>MSGSEELLEELRELLERLQELLELIEQGKITPEQLREAIALLIEVLQILYEALRELAEQLQRLREELGS[2x]

Here, we computationally designed monomeric and homo-oligomeric miniproteins binding with high affinity to the MERS-CoV spike (S) glycoprotein, the main target of neutralizing antibodies and vaccine development. MERS-CoV S comprises an S1 subunit, which mediates binding to sialosides via the N-terminal domain (NTD) and to the dipeptidyl-peptidase 4 entry receptor (DPP4) via the receptor-binding domain (RBD), as well as an S2 subunit which promotes virus and host membrane fusion to initiate infection,12–17. We show that these miniproteins broadly neutralize a panel of MERS-CoV S variants, spanning the known antigenic diversity of this pathogen, by targeting a conserved site in the receptor-binding domain (RBD). The miniproteins directly compete with binding of the DPP4 receptor to MERS-CoV S, thereby blocking viral attachment to the host entry receptor and subsequent membrane fusion.

Based on our previous success in designing a homotrimeric, pan-variant SARS-CoV-2 inhibitor, designated TRI2–224–27, we set out to engineer homotrimeric versions of cb3 to enable simultaneous engagement of all three RBDs within a MERS-CoV S trimer and enhance potency and breadth further through avidity. 12 trimeric cb3 constructs were designed, consisting of 6 oligomerization domains with both N- and C-terminal fusions for each oligomerization domain (denoted with prefix ‘n’ or ‘c’ to describe the position of the miniprotein relative to the trimerization domain). Two of these failed to express (nTrimer3 and nTrimer4). Evaluation of neutralizing activity against the MERS-CoV EMC/2012, Jordan/2012 and United Kingdom/2012 pseudoviruses revealed that trimeric cb3 miniproteins were endowed with at least an order of magnitude greater potency, compared to monomeric cb3, with the exception of cTrimer1, cTrimer3, cTrimer4, cTrimer5 and cTrimer6 fusions which failed to neutralize MERS-CoV United Kingdom/2012 S VSV pseudotypes (full curves for each replicate in Fig S1).>[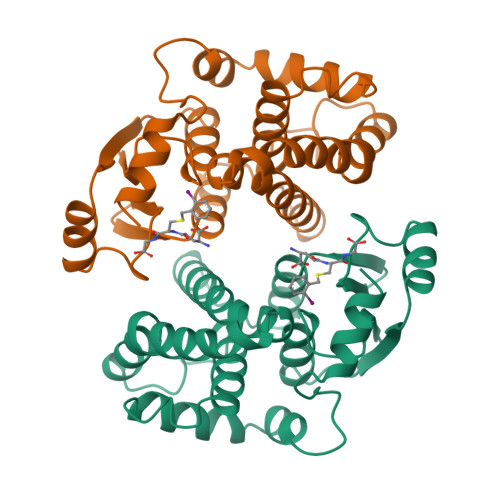8x]MAARPKLHYPNGRGRMESVRWVLAAAGVEFDEEFLETKEQLYKLQDGNHLLFQQVPMVEIDGMKLVQTRSILHYIADKHNLFGKNLKERTLIDMYVEGTLDLLELLIMHPFLKPDDQQKEVVNMAQKAIIRYFPVFEKILRGHGQSFLVGNQLSLADVILLQTILALEEKIPNILSAFPFLQEYTVKLSNIPTIKRFLEPGSKKKPPPDEIYVRTVYNIFRP>MRGSHHHHHH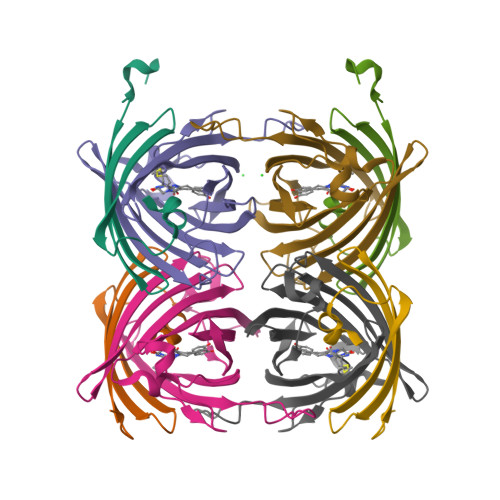GSASFLKKTMPFKTTIEGTVNGHYFKCTGKGEGNPFEGTQEMKIEVIEGGPLPFAFHILSTSC[2x];>[2x]MYGSKTFIKYVSGIPDYFKQSFPEGFTWERTTTYEDGGFLTAHQDTSLDGDCLVYKVKILGNNFPADGPVMQNKAGRWEPSTEIVYEVDGVLRGQSLMALKCPGGRHLTCHLHTTYRSKKPASALKMPGFHFEDHRIEIMEEVEKGKCYKQYEAAVGRYCDAAPSKLGHN Type I RM enzymes house these activities in a multisubunit complex having ATP-dependent translocation activity that pulls thousands of duplex DNA base pairs through the stationary enzyme, eventually cleaving at random sites distant from the recognition site. Upon identification of an unmethylated specific DNA sequence, two HsdR motor subunits, which bear the endonuclease and ATP-dependent DNA translocation activities in the fully assembled DNA-HsdS-HsdM2-HsdR2 complex, start to translocate the duplex DNA toward the stationary enzyme from both directions, producing two extruded DNA loops flanking the enzyme complex. The X-ray crystal structure of the HsdR subunit with bound ATP from the Type I restriction enzyme of E. coli plasmid R124 revealed four structural and functional domains forming a planar array: one nuclease domain of PD-(E/D)xK type that houses three endonuclease active-site residues and a QxxxY motif common to the RecB-like nucleases; two RecA-like helicase domains of SF2 type that use ATP to translocate duplex DNA without unwinding; and a C-terminal α-helix-rich domain presumed to contact the HsdS-HsdM2 methylase. ATP bound between the two helicase domains was found unexpectedly to also contact Lys220 of the endonuclease domain, suggesting a means by which nuclease and translocation activities might communicate.

The three mutant HsdR subunits were crystallized with bound ATP, and their X-ray crystal structures were refined at 2.74 Å, 2.84 Å, and 2.99 Å for the Lys220Arg, Lys220Ala, and Lys220Glu mutants, respectively, guided by the higher-resolution structure of the WT HsdR-ATP complex (2.6 Å; 22). The crystallization conditions used previously for WT HsdR yielded crystals only for the Lys220Arg mutant; the Lys220Ala and Lys220Glu mutants required altered conditions. In the Lys220Arg mutant the ε-NH nitrogen atom lies 3.7 Å from adenine N3, bringing its proton almost to hydrogen-bonding distance with the base edge. The closer of the two equivalent ω-NH2 nitrogens lies 3.1 Å from ribose 3'-OH and 2.6 Å from ribose 2'-OH, enabling one or more potential hydrogen bonds with the ribose. Thus, Arg substitutes structurally for the Lys220 interaction with the ATP base edge, and can make a novel interaction with the ribose as well. Residue 220 is located at the base of a loop made by residues 215–219 that is well-resolved only in the WT and Lys220Arg mutant structures. In the WT and Lys220Arg structures, where residue 220 contacts ATP, Asn221 points away from ATP. In the WT HsdR structure the backbone and sidechains of residues 182–190 are unresolved; in the Lys220Glu mutant residues 181–191 are unresolved; and in the Lys220Arg mutant residues 181–188 are unresolved. The crystal structures reported here show that mutant Lys220Arg HsdR maintains contact to ATP similarly as does Lys220 of WT HsdR, whereas mutants Lys220Ala and Lys220Glu lose contact with ATP.

>[2x]MTHQTHTIAESNNFIVLDKYIKAEPTGDSYQSESDLERELIQDLRNQGYEFISVKSQSAMLANVREQLQNLNGVVFNDSEWRRFTEQYLDNPSDGILDKTRKIHIDYICDFIFDDERLENIYLIDKKNLMRNKVQIIQQFEQAGSHANRYDVTILVNGLPLVQIELKKRGVAIREAFNQIHRYSKESFNSENSLFKYLQLFVISNGTDTRYFANTTKRDRNSFDFTMNWAKSDNTLIKDLKDFTATCFQKHTLLNVLVNYSVFDSSQTLLVMRPYQIAATERILWKIKSSFTAKNWSKPESGGYIWHTTGSGKTLTSFKAARLATELDFIDKVFFVVDRKDLDYQTMKEYQRFSPDSVNGSENTAGLKRNLDKDDNKIIVTTIQKLNNLMKAESDLPVYNQQVVFIFDECHRSQFGEAQKNLKKKFKRYYQFGFTGTPIFPENALGSETTASVFGRELHSYVITDAIRDEKVLKFKVDYNDVRPQFKSLETETDEKKLSAAENQQAFLHPMRIQEITQYILNNFRQKTHRTFPGSKGFNAMLAVSSVDAAKAYYATFKRLQEEAANKSATYKPLRIATIFSFAANEEQNAIGEISDETFDTSAMDSSAKEFLDAAIREYNSHFKTNFSTDSNGFQNYYRDLAQRVKNQDIDLLIVVGMFLTGFDAPTLNTLFVDKNLRYHGLMQAFSRTNRIYDATKTFGNIVTFRDLERSTIDAITLFGDKNTKNVVLEKSYTEYMEGFTDAATGEAKRGFMTVVSELEQRFPDPTSIESEKEKKDFVKLFGEYLRAENILQNYDEFATLKALQQIDLSDPVAVEKFKAEHYVDDEKFAELQTIRLPADRKIQDYRSAYNDIRDWQRREKEAEKKEKSTTDWDDVVFEVDLLKSQEINLDYILGLIFEHNRQNKGKGEMIEEVKRLIRSSLGNRAKEGLVVDFIQQTNLDDLPDKASIIDAFFTFAQREQQREAEALIKEENLNEDAAKRYIRTSLKREYATENGTELNETLPKLSPLNPQYKTKKQAVFQKIVSFIEKFKGVGGKI IadA is a binuclear metalloenzyme and a member of the amidohydrolase superfamily. This enzyme catalyzes the hydrolytic cleavage of β-aspartyl dipeptides. In the present study, we determined the crystal structures of IadA from Colwellia psychrerythraea strain 34H (CpsIadA) in its ligand-free form and that in complex with β-isoaspartyl lysine, and subsequently characterized its enzymatic properties. The CpsIadA monomer structure contains ten α-helices and eighteen β-strands, and the overall structure is divided into two distinct domains (a β-sandwich domain and a catalytic domain).

The E80Q mutant had no catalytic activity toward β-Asp-Leu, but its CD spectra and denaturation temperature (Tm) were similar to WT, indicating that this mutation affected catalytic activity but not the overall folding and integrity of CpsIadA. A structural comparison between the ligand-free wild type CpsIadA structure and the structure of the CpsIadA E80Q mutant complexed with β-isoaspartyl lysine show several structural changes occur upon ligand binding. Notably, upon substrate binding, a slight tilt of residue Tyr140 is observed with a 61° rotation. Tyr140 interacts with the O04 and O07 atoms of the bound β-isoaspartyl lysine. The bound β-isoaspartyl lysine, with the exception of the lysine side-chain region, forms tight interactions with CpsIadA. In detail, the O07 atom of the bound β-isoaspartyl lysine interacts with the ZN1 metal ion. The OG1 atom of Thr109 and the OE1 atom of Glu80 interact with the N11 atom of the β-isoaspartyl lysine, and the SG atom of Cys297 interacts with the O13 atom of β-isoaspartyl lysine. Residues Arg173 and Arg237 interact with the O01 and O04 atoms of the β-isoaspartyl lysine. The lysine side chain of β-isoaspartyl lysine did not have any specific interactions with CpsIadA. Thus, this region has a relatively weak electron density. These results suggest that the side chain of the second amino acid in β-the isoaspartyl substrate is not critical for ligand recognition and specificity.

>[2x]MNDSQTMLILLCNVNIYAPNPLGIKDVLIAGNKIAAIYDHGQGEITIPKQWPVKVINFDGAILTPGFIDSHAHITGGGGQAGFATQVPPVGLTEFTHAGVTTVVGLLGTDDTTRSTENLLSRVYGLREEGLSAYCWTGGYHFPLTTITGSAKSDIAFLEPVIGIGEFAISDHRSSQPTFEEVIRLASETHVAGLITGKAGVIHFHLGDGERRLELIERAIRETELPARVFNPTHVNRNKPLFEDSCKLLSKGCHIDLTAFPAGTAQPGWEACDAIEMAVERQLPLEQITLSSDGGGCLPCFDPQGELQHMDFGRASTLGETLVATLNKGLSLETVLPMLTSNVANILRFKNKGQIAVGFDADLLVMNEKYEITDVMAQGVWHKQNNQTMIKGTFE>MYVCHFENCGKAFKKHNQLKVHQFSHTQQLPYECPHEGCDKRFSLPSRLKRHEKVHAGYPCKKDDSCSFVGKTWTL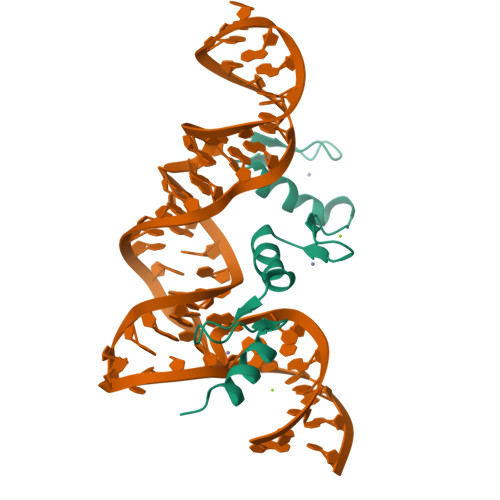YLKHVAECHQD[3x]>[8x]AAGCQVLWGVNQWNTGFTANVTVQNTSSAPVQGW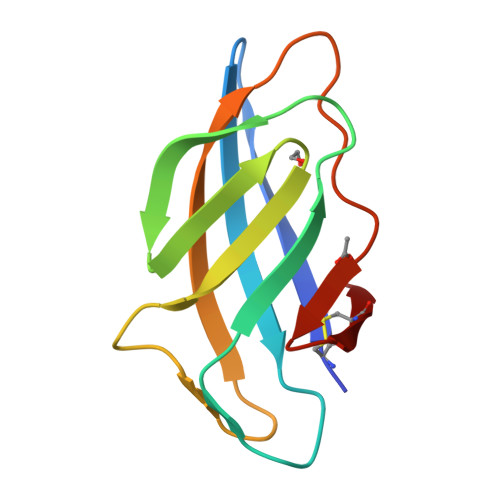TLTFSFPSGQQVTQAWSSTVTQSGSAVTVQNAPWNGSIPAGGTAQFGFNGSWTGTNAAPTAFSLNGTPCTVG> EELH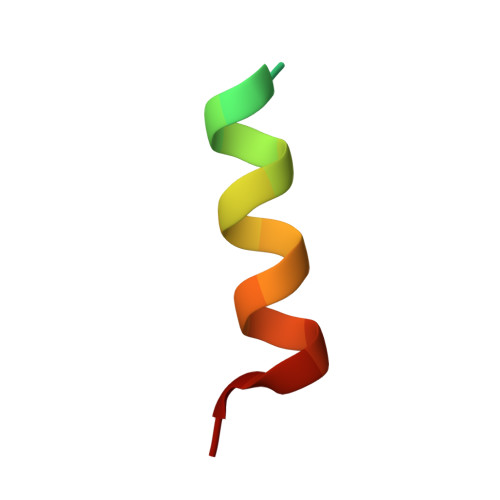SLDPRRQELLEARFTGV> GHSNRQVQLMARQQRLKAIEDRLEKFYIPLIKAFSSYV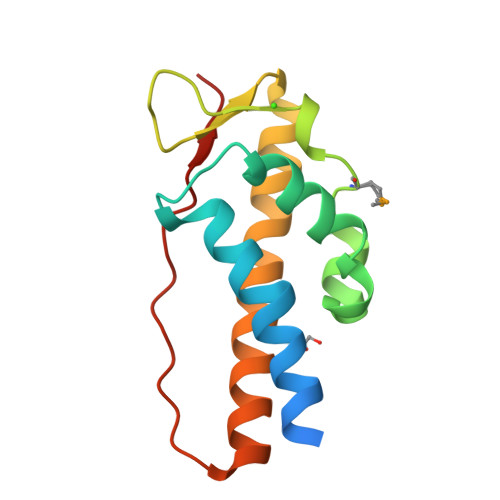YTAQTEDEIETIITCRRYLAGNNLLRVLPMHFKFKADKIAGSANWTFYAKEDFEQWKEALDVLWEEFLEVLKEYYTLSGTEISLPEKPDWLIGYKGS>SEKYFVKNGQPHFLISGEVHYFRINPKLWRNHLQLLKQTGADTVSTYIPWDWHEIEEDDFDFEGKTHPARNLIRFIKLCKEENLDLIVKPGPYILAEYENQGLPSWLLKKLSKNAFALDENGNVISPDLVSYLSDEFLEYTFKWYDKVMPIISKHQKEHYGPITMMQLCNEIGVFQWLSGKSDYNPKVINLYKEFIIQRYKTIEKLNSVYSTNYNSFDDLKAPSGKIKLRSDYCAYFDFHLFFREYYNKYISILKNKIRSFGINIKLTHNIPGWIYGNASELPMLISTYSEIMKNHPDIIFGLDHIPEFVSFRNAHSDLACNKILEAMQPEAPVWAAEFQAGTREHHVKAYAKDLETFYIASLAHGIKGFNYYMFSQGINPEGKGFYGKTFYFQTALDAASNKLALYDSIKKVNRFIRKEQKDLLRTNVNSEICVGFYKPY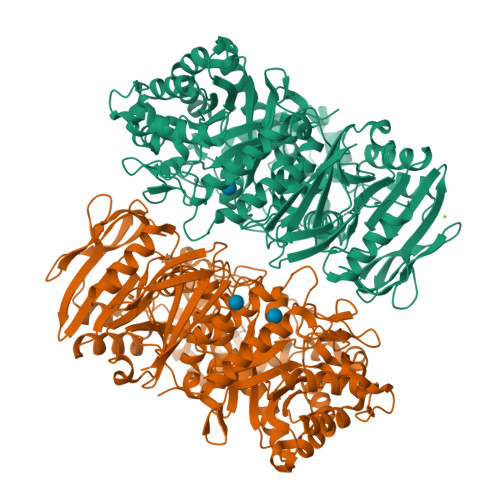FFTELISSQLLKEKKLNVEELGLYIDPRFLREEILFNGLLRGLQTLNYNYDVVDLENCDLKSLTAYKQLWITSAEFMDAETQNLLSEFVLNGGNLILYPAVPTLDNYLNRCEILKNNFGIEFITKDSSHKVSAFGIEDVFTAFSKKQIYNDTNSKPIAFTQENEICGIRKKIGKGELTILGFAFGYTSDEHLELIDKLVKLNKIKRELFVSDKDIQFVVRENNKSRYIFFLNYHNERKTFNYRKSSELKKKKSEEISIAPFSYKVIKENK[2x]> MNITKPFPLPTGYFGIPLGLAALSLAWFHLENLFPAARMVSDVLGIVASAVWILFILMYAYKLRYYFEEVRAEYHSPVRFSFIALIPITTMLVGDILYRWNPLIAEVLIWIGTIGQLLFSTLRVSELWQGGVFEQKSTHPSFYLPAVA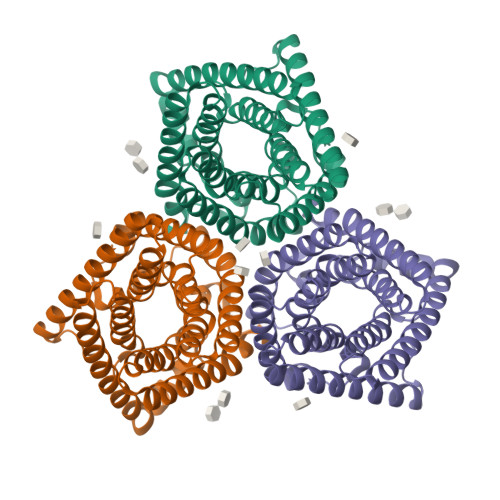ANFTSASSLALLGYHDLGYLFFGAGMIAWIIFEPVLLQHLRISSLEPQFRATMGIVLAPAFVCVSAYLSINHGEVDTLAKILWGYGFLQLFFLLRLFPWIVEKGLNIGLWAFSLGLASMANSATAFYHGNVLQGVSIFAFVFSNVMIGLLVLMTIYKLTKGQFFLK>MIPRVFIYRLPQDDPRKNTAIKLVRFGFAQLVDSIKALPSGSIILDPTVKTPLTPSDRVIAESRGLSLIDCSWKRAVDVHTKFIRGKFIRRRLPLLIAANPTHYGKPYILSTIEAVAAALYIMGFKD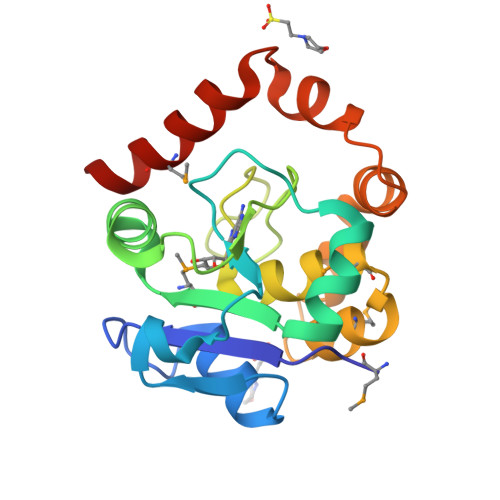EAMEVLRLYKWGPNFIIINQKYLERYAAGDLSPERELLGVDDVDNGLEQLMRVLTNGD[3x]>[2x]GSHMQLTAAQELMIQQLVAAQLQCNKRSFSDQPKVTPWPLGADPQSRDARQQRFAHFTELAIISVQEIVDFAKQVPGFLQLGREDQIALLKASTIEIMLLETARRYNHETECITFLKDFTYSKDDFHRAGLQVEFINPIFEFSRAMRRL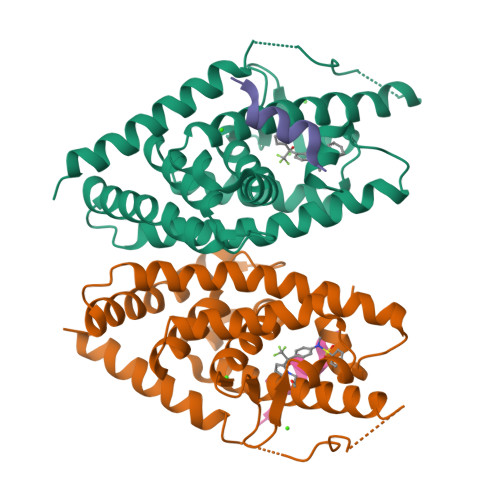GLDDAEYALLIAINIFSADRPNVQEPGRVEALQQPYVEALLSYTRIKRPQDQLRFPRMLMKLVSLRTLSSVHSEQVFALRLQDKKLPPLLSEIWDVHE;>DHQLLRYLLDKD[2x]>MSKLVLTGERHYTRNDDIRQSILALGEPGTFMTQDVNIIQTQIEQRLPWIKQVSVRKQWPDELKIHLVEYVPIARWNDQHMVDAEGNTFSVPPERTSKQVLPMLYGPEGSANEVLQGYREMGQMLAKDRFTLKEAAMTARRSWQLTLNNDIKLNLGRGDTMKRLARFVELYPVLQQQAQTDGKRISYVDLRYDSGAAVGWAPLPPEESTQQQNQAQAEQQGSHHHHHH[2x];>QEALEERARNELSLTRPGETFYRL[2x]

In Gram-negative Escherichia coli bacteria, FtsZ recruits cytosolic, transmembrane, periplasmic, and outer membrane proteins, assembling the divisome that facilitates bacterial cell division. One such divisome component, FtsQ, a bitopic membrane protein with a globular domain in the periplasm, has been shown to interact with many other divisome proteins. FtsB and FtsL are small bitopic inner membrane proteins (103 and 121 residues in E. coli, respectively). Previously, the structure of the periplasmic domain of FtsQ from E. coli has been solved by X-ray crystallography and shown to consist of two subdomains, named α and β.

Our crystal structure of FtsB bound to the β domain of FtsQ shows that only residues 64 to 87 of FtsB interact with FtsQ. A synthetic peptide comprising those 24 FtsB residues recapitulates the FtsQ-FtsB interactions. The structure of the complex between the periplasmic domains of E. coli FtsB and FtsQ contained FtsB residues 64 to 87 only. We showed that this subdomain is indeed necessary for the interaction but is also sufficient, suggesting that the remaining residues within FtsB are disordered in the crystals and do not bind to FtsQ. In accordance with these data, it has been shown that FtsB truncated at Y85 is unable to complement and interact with FtsQ, whereas FtsB truncated at D90 is fully functional, and this is also supported by our data showing that FtsB 64–88 binds as well as the entire periplasmic domain comprising residues 22 to 103. FtsB forms a helix, followed by a linker largely in β-strand conformation, leading to the final β-strand that extends the central β-sheet of the FtsQ β domain by binding to its last β-strand. The only helix resolved in FtsB, approximately residues 65 to 75, makes a number of charged interactions with the rest of FtsB and FtsQ, most notably two salt bridges that may be involved in stabilizing FtsB’s conformation (E68-R79 and R72-E82). Both salt bridges are also involved in binding to FtsQ via D245 and R247. In the FtsQ-FtsB structure, FtsB Y85 is oriented toward FtsQ L226, a position that was previously shown to cross-link very strongly to FtsB. The complex represents an exciting target for structure-based design of protein interaction inhibitors shutting down cell division based on peptides or peptide mimetics, as the FtsQ-FtsB interaction surface is small, the 64–87 FtsB peptide is water soluble, and the interaction is easily interrupted by single mutations.> ATCDDGRTTANAACCILFPILDDIQENLFDGAQCGEEVHESLRLTFHDAIGFSPTLGGGGADGSIIAFDTIETNFPANAGIDEIVSAQKPFVAKHNISAGDFIQFAGAVGVSNCPGGVRIPFFLGRPDAVAASPDHLVPEPFDSVDSILARMGDAGFSPVEVVWLLASHSIAAAAKVDPSIPGTPFDSTPGVFDSQFFIETQLKGRLFPGTADNKGEAQSPLQGEIRLQSDH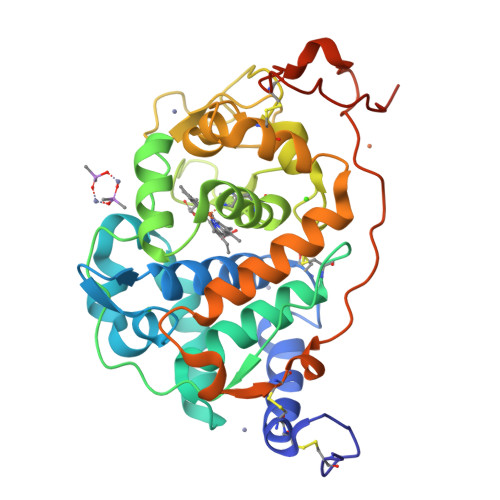LLARDPQTACEWQSMVNNQPKIQNRFAATMSKMALLGQDKTKLIDCSDVIPTPPALVGAAHLPAGFSLSDVEQACAATPFPALTADPGPVTSVPPVPGS> X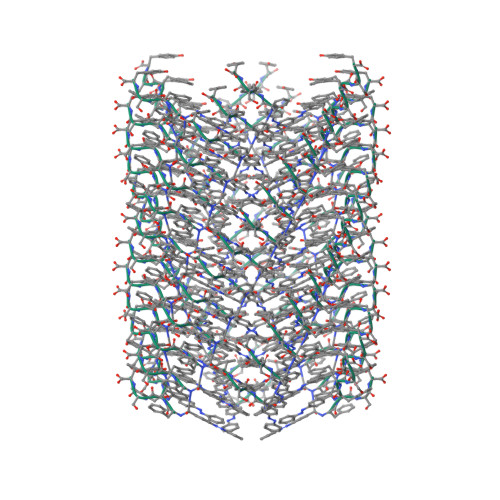FFSY> MHHHHHHSSGMSWTVDIPKEVLPDLPPLPEGMQQQFEDTISRDAKQQPTWDRAQAENVRKILESVPPIVVAPEVLELKQKLADVANGKAFLLQGGDCAETFESNTEPHIRANVKTLLQMAVVLTYGASTPVIKMARIAGQYAKPRSSDLDGNGLPNYRGDIVNGVEATPEARRHDPARMIRAYANASAAMNLVRALTSSGTADLYRLSEW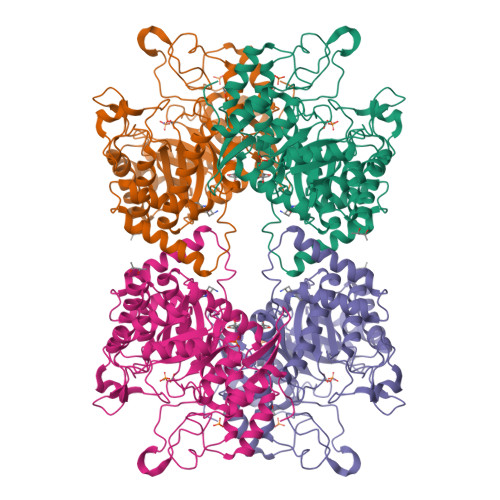NREFVANSPAGARYEALAREIDSGLRFMEACGVSDESLRAADIYCSHEALLVDYERSMLRLATDEEGNEELYDLSAHQLWIGERTRGMDDFHVNFASMISNPIGIKIGPGITPEEAVAYADKLDPNFEPGRLTIVARMGHDKVRSVLPGVIQAVEASGHKVIWQSDPMHGNTFTASNGYKTRHFDKVIDEVQGFFEVHRALGTHPGGIHIEFTGEDVTECLGGAEDITDVDLPGRYESACDPRLNTQQSLELAFLVAEMLRN> MTVVPENFVPGLDGVVAFTTEIAEPDKDGGALRYRGVDIEDLVSQRVTFGDVWALLVDGNFGSGLPPAEPFPLPIHSGDVRVDVQAGLAMLAPIWGYAPLLDIDDATARQQLARASVMALSYVAQSARGIYQPAVPQRIIDEWSTVTARFMTRWQGEPDPRHIEAIDAYWVSAAEHGMNASTFTARVIASTGADVAAALSGAIGAMSGPLHGGAPARVLPM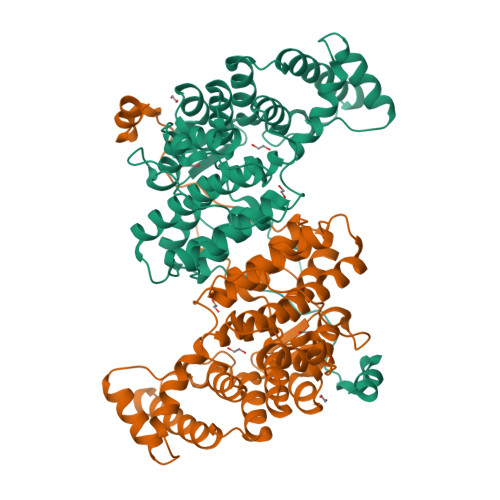LDEVERAGDARSVVKGILDRGEKLMGFGHRVYRAEDPRARVLRAAAERLGAPRYEVAVAVEQAALSELRERRPDRAIETNVEFWAAVVLDFARVPANMMPAMFTCGRTAGWCAHILEQKRLGKLVRPSAIYVGPGPRSPESVDGWERVLTTAHHHHHH> SDRVLQLKLGNSAIVTQEAANMCCAYGEWPSYLPDNEATAIDKPTQPETSTDRFYTLKSVKWEGTSTGWWWKLPDALNQTGMFGQNVQYHYLYRSGFLCHVQCNATKFHQGALLVVAIPEHQLGKYNTGTSASFDDVMKGKTGGVFT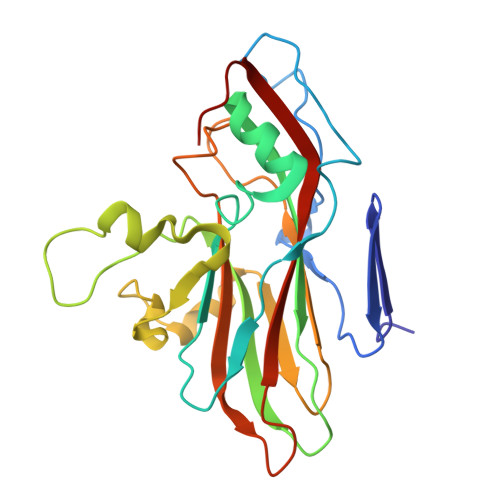HPYVLDDGTSLACSLIFPHQWINLRTNNSATIMLPWMNCAPMDFALRHNQWTLAIIPVVPLNTSGGTTMVPITVSIAPMCCEFNGLRNAIT>[2x]SNATFEEDDNMERAAVTGIAFDKNQARINVRGVPDKPGVAYQILG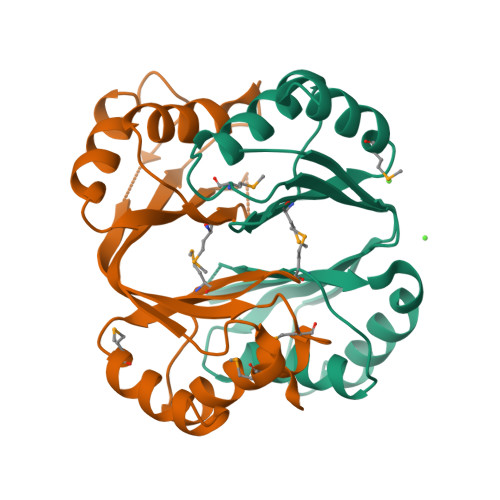AVADANIEVDMIIQNVGSEGTTDFSFTVPRGDYKQTLEILSERQDSIGAASIDGDDTVCKVSAVGLGMRSHVGVAAKIFRTLAEEGINIQMISTSEIKVSVLIDEKYMELATRVLHKAFNLG>[3x]MSSDATLVDTVNASQSRQVFWDEDVYALEIERIFSRAWLMLGHESLVPKPGDFITTYMAEDKVILSHQSDGTFRAFINSCSHRGNQICHADSGNAKAFVCNYHGWVFGQDGSLVDVPLESRCYHNSLDKQKLAAKSVRVETYKGFIFGCHDPEAPSLEDYLGEFRYYLDTIWEGAGGGMELLGPPMKSLLQCNWKVPAENFIGDGYHVGWTHAAALSQIGGELAGLAGNRADIPFDDLGLQFTTRHGHGFGVIDNAAAGLHIKREGWTKFLEDTRGEVRRKFGPERERLYLGHWNCSIFPNCSFLYGTNTFKIWHPRGPHEIEVWTYTIVPRDADPATKSMIQREAIRTFGTAGTLESDDGENMSSATYINRGVITRNGRMNSTMGVGYEGPHPVYPGIVGISFIGETSYRGFYRFWKEMIDAPDWASVKANDDTWDSVFPNRNFWNEKLNAAE;>[3x]MSSEQIPVTPDVHYDIEAHYRAEVRMFQTGQYREWLQGMVAEDIHYWMPIYEQRLTRDRRPDPTPDDAAIYNDDFGELKQRVERLYSGQVWMEDPPSKIRYFVSNVEAFEAGNGELDVLSNILVYRNRRQTEVTVHTLGREDKLRRDGNGFKVFRRKLILDARVTQDKNLYFFC

The initial step involved in oxidative hydroxylation of monoaromatic and polyaromatic compounds by the microorganism Sphingobium yanoikuyae strain B1 (B1), previously known as Sphingomonas yanoikuyae strain B1 and Beijerinckia sp. strain B1, is performed by a set of multiple terminal Rieske non-heme iron oxygenases. These enzymes share a single electron donor system consisting of a reductase and a ferredoxin (BPDO-FB1). One of the terminal Rieske oxygenases, biphenyl 2,3-dioxygenase (BPDO-OB1), is responsible for B1's ability to dihydroxylate large aromatic compounds, such as chrysene and benzo[a]pyrene. Rieske oxygenase systems have multiple components whose function is to transfer electrons from NAD(P)H to active molecular oxygen and ultimately oxidize aromatic hydrocarbon substrates.

The asymmetric unit contains the entire BPDO-OB1α3β3 hexamer and residues 6 – 454 of the α subunits and residues 5 – 174 of the β subunits were modeled into the electron density. The structure has been refined to a resolution of 1.7 Å with a final Rfactor of 18.8 % and an Rfree of 22.9 %. The three copies of the α and β subunits form an α3β3 quaternary structure similar to the quaternary structure observed in all known RO structures. The hexamer forms a mushroom-shaped structure, illustrated in Figure 1, where the three α subunits form the cap and the three β subunits form the stem. The loop region located at the entrance of the α subunit active site is disordered, with higher than average B-factors and low side-chain electron density. The mononuclear iron is coordinated by two histidines, His-207 and His-212, and one aspartate, Asp-360, at the rear of the active site. In BPDO-OB1, a clear bimodal electron density distribution was not observed, but instead an egg-shaped electron density above the mononuclear iron was present. Residual positive electron density was not observed on the Fo-Fc electron density maps when modeling molecular oxygen as the fourth iron ligand; however, refinement with relaxed restraints (refinement restraints allowing the oxygen-oxygen bond an RMSD of 0.3Å) placed the oxygen-oxygen bond distance at 0.8 – 1.1Å in the three subunits. The final model has both molecular oxygen and water bound to the iron in partially occupied states. The BPDO-OB1 crystals were grown in atmospheric conditions, therefore molecular oxygen or water could constitute the fourth ligand on the mononuclear iron.>MACLSRIDANLLQYYEKPEPNNTVDLYVSNNSNNNGLKEGDKSISTPVPQPYGSEYSNCLLLSNSEYICYHFSSRSTLLTFYPLSDAYHGKTINIHLPNASMNQRYTLTIQEVEQQLLVNVILKDGSFLTLQLPLSFLFSSANTLNGEWFHLQNPYDFTVRVPHFLFYVSPQFSVVFLEDGGLLGLKKVDGVHYEPLLFNDNSYLKSLTRFFSRSSKSDYDSVISCKLFHERYLIVLTQNCHLKIWDLTSFTLIQDYDMVSQSDSDPSHFRKVEAVGEYLSLYNNTLVTLLPLENGLFQMGTLLVDSSGILTYTFQNNIPTNLSASAIWSIVDLVLTRPLELNVEASYLNLIVLWKSGTASKLQILNVNDESFKNYEWIESVNKSLVDLQSEHDLDIVTKTGDVERGFCNLKSRYGTQIFERAQQILSENKIIMAHNEDEEYLANLETILRDVKTAFNEASSITLYGDEIILVNCFQPYNHSLYKLNTTVENWFYNMHSETDGSELFKYLRTLNGFASTLSNDVLRSISKKFLDIITGELPDSMTTVEKFTDIFKNCLENQFEITNLKILFDELNSFDIPVVLNDLINNQMKPGIFWKKDFISAIKFDGFTSIISLESLHQLLSIHYRITLQVLLTFVLFDLDTEIFGQHISTLLDLHYKQFLLLNLYRQDKCLLAEVLLKDSSEFSFGVKFFNYGQLIAYIDSLNSNVYNASITENSFFMTFFRSYIIENTSHKNIRFFLENVECPFYLRHNEVQEFMFAMTLFSCGNFDQSYEIFQLHDYPEAINDKLPTFLEDLKSENYHGDSIWKDLLCTFTVPYRHSAFYYQLSLLFDRNNSQEFALKCISKSAEYSLKEIQIEELQDFKEKQHIHYLNLLIHFRMFEEVLDVLRLGHECLSDTVRTNFLQLLLQEDIYSRDFFSTLLRLCNAHSDNGELYLRTVDIKIVDSILSQNLRSGDWECFKKLYCFRMLNKSERAAAEVLYQYILMQADLDVIRKRKCYLMVINVLSSFDSAYDQWILNGSKVVTLTDLRDELRGL[2x];>MTIDDSNRLLMDVDQFDFLDDGTAQLSNNKTDEEEQLYKRDPVSGAILVPMTVNDQPIEKNGDKMPLKFKLGPLSYQNMAFITAKDKYKLYPVRIPRLDTSKEFSAYVSGLFEIYRDLGDDRVFNVPTIGVVNSNFAKEHNATVNLAMEAILNELEVFIGRVKDQDGRVNRFYELEESLTVLNCLRTMYFILDGQDVEENRSEFIESLLNWINRSDGEPDEEYIEQVFSVKDSTAGKKVFETQYFWKLLNQLVLRGLLSQAIGCIERSDLLPYLSDTCAVSFDAVSDSIELLKQYPKDSSSTFREWKNLVLKLSQAFGSSATDISGELRDYIEDFLLVIGGNQRKILQYSRTWYESFCGFLLYYIPSLELSAEYLQMSLEANVVDITNDWEQPCVDIISGKIHSILPVMESLDSCTAAFTAMICEAKGLIENIFEGEKNSDDYSNEDNEMLEDLFSYRNGMASYMLNSFAFELCSLGDKELWPVAIGLIALSATGTRSAKKMVIAELLPHYPFVTNDDIEWMLSICVEWRLPEIAKEIYTTLGNQMLSAHNIIESIANFSRAGKYELVKSYSWLLFEASCMEGQKLDDPVLNAIVSKNSPAEDDVIIPQDILDCVVTNSMRQTLAPYAVLSQFYELRDREDWGQALRLLLLLIEFPYLPKHYLVLLVAKFLYPIFLLDDKKLMDEDSVATVIEVIETKWDDADEKSSNLYETIIEADKSLPSSMATLLKNLRKKLNFKLCQAFM[2x];>MFNKSVNSGFTFGNQNTSTPTSTPAQPSSSLQFPQKSTGLFGNVNVNANTSTPSPSGGLFNANSNANSISQQPANNSLFGNKPAQPSGGLFGATNNTTSKSAGSLFGNNNATANSTGSTGLFSGSNNIASSTQNGGLFGNSNNNNITSTTQNGGLFGKPTTTPAGAGGLFGNSSSTNSTTGLFGSNNTQSSTGIFGQKPGASTTGGLFGNNGASFPRSGETTGTMSTNPYGINISNVPMAVADMPRSITSSLSDVNGKSDAEPKPIENRRTYSFSSSVSGNAPLPLASQSSLVSRLSTRLKATQKSTSPNEIFSPSYSKPWLNGAGSAPLVDDFFSSKMTSLAPNENSIFPQNGFNFLSSQRADLTELRKLKIDSNRSAAKKLKLLSGTPAITKKHMQDEQDSSENEPIANADSVTNIDRKENRDNNLDNTYLNGKEQSNNLNKQDGENTLQHEKSSSFGYWCSPSPEQLERLSLKQLAAVSNFVIGRRGYGCITFQHDVDLTAFTKSFREELFGKIVIFRSSKTVEVYPDEATKPMIGHGLNVPAIITLENVYPVDKKTKKPMKDTTKFAEFQVFDRKLRSMREMNYISYNPFGGTWTFKVNHFSIWGLVNEEDAEIDEDDLSKQEDGGEQPLRKVRTLAQSKPSDKEVILKTDGTFGTLSGKDDSIVEEKAYEPDLSDADFEGIEASPKLDVSKDWVEQLILAGSSLRSVFATSKEFDGPCQNEIDLLFSECNDEIDNAKLIMKERRFTASYTFAKFSTGSMLLTKDIVGKSGVSIKRLPTELQRKFLFDDVYLDKEIEKVTIEARKSNPYPQISESSLLFKDALDYMEKTSSDYNLWKLSSILFDPVSYPYKTDNDQVKMALLKKERHCRLTSWIVSQIGPEIEEKIRNSSNEIEQIFLYLLLNDVVRASKLAIESKNGHLSVLISYLGSNDPRIRDLAELQLQKWSTGGCSIDKNISKIYKLLSGSPFEGLFSLKELESEFSWLCLLNLTLCYGQIDEYSLESLVQSHLDKFSLPYDDPIGVIFQLYAANENTEKLYKEVRQRTNALDVQFCWYLIQTLRFNGTRVFSKETSDEATFAFAAQLEFAQLHGHSLFVSCFLNDDKAAEDTIKRLVMREITLLRASTNDHILNRLKIPSQLIFNAQALKDRYEGNYLSEVQNLLLGSSYDLAEMAIVTSLGPRLLLSNNPVQNNELKTLREILNEFPDSERDKWSVSINVFEVYLKLVLDNVETQETIDSLISGMKIFYDQYKHCREVAACCNVMSQEIVSKILEKNNPSIGDSKAKLLELPLGQPEKAYLRGEFAQDLMKCTYKI[2x];>MVVIANAHNELIHDAVLDYYGKRLATCSSDKTIKIFEVEGETHKLIDTLTGHEGPVWRVDWAHPKFGTILASCSYDGKVLIWKEENGRWSQIAVHAVHSASVNSVQWAPHEYGPLLLVASSDGKVSVVEFKENGTTSPIIIDAHAIGVNSASWAPATIEEDGEHNGTKESRKFVTGGADNLVKIWKYNSDAQTYVLESTLEGHSDWVRDVAWSPTVLLRSYLASVSQDRTCIIWTQDNEQGPWKKTLLKEEKFPDVLWRASWSLSGNVLALSGGDNKVTLWKENLEGKWEPAGEVHQ[2x];>[2x]MQPFDSGHDDLVHDVVYDFYGRHVATCSSDQHIKVFKLDKDTSNWELSDSWRAHDSSIVAIDWASPEYGRIIASASYDKTVKLWEEDPDQEECSGRRWNKLCTLNDSKGSLYSVKFAPAHLGLKLACLGNDGILRLYDALEPSDLRSWTLTSEMKVLSIPPANHLQSDFCLSWCPSRFSPEKLAVSALEQAIIYQRGKDGKLHVAAKLPGHKSLIRSISWAPSIGRWYQLIATGCKDGRIRIFKITEKNLQVELLSEHDDHNGEVWSVSWNLTGTILSSAGDDGKVRLWKATYSNEFKCMSVITAQQ;>MELSPTYQTERFTKFSDTLKEFKIEQNNEQNPIDPFNIIREFRSAAGQLALDLANSGDESNVISSKDWELEARFWHLVELLLVFRNADLDLDEMELHPYNSRGLFEKKLMQDNKQLYQIWIVMVWLKENTYVMERPKNVPTSKWLNSITSGGLKSCDLDFPLRENTNVLDVKDKEEDHIFFKYIYELILAGAIDEALEEAKLSDNISICMILCGIQEYLNPVIDTQIANEFNTQQGIKKHSLWRRTVYSLSQQAGLDPYERAIYSYLSGAIPNQEVLQYSDWESDLHIHLNQILQTEIENYLLENNQVGTDELILPLPSHALTVQEVLNRVASRHPSESEHPIRVLMASVILDSLPSVIHSSVEMLLDVVKGTEASNDIIDKPYLLRIVTHLAICLDIINPGSVEEVDKSKLITTYISLLKLQGLYENIPIYATFLNESDCLEACSFILSSLEDPQVRKKQIETINFLRLPASNILRRTTQRVFDETEQEYSPSNEISISFDVNNIDMHLIYGVEWLIEGKLYVDAVHSIIALSRRFLLNGRVKALEQFMERNNIGEICKNYELEKIADNISKDENEDQFLEEITQYEHLIKGIREYEEWQKSVSLLSSESNIPTLIEKLQGFSKDTFELIKTFLVDLTSSNFADSADYEILYEIRALYTPFLLMELHKKLVEAAKLLKIPKFISEALAFTSLVANENDKIYLLFQSSGKLKEYLDLVARTATLSN[2x];>[2x]MSEKKVHLRLRKELSVPIAVVENESLAQLSYEEESQASLMDISMEQQQLRLHSHFDNSKVFTENNRYIVKTLQTDYSSGFSNDDELNGYIDMQIGYGLVNDHKKVYIWNIHSTQKDTPYITVPFRSDDNDEIAVAPRCI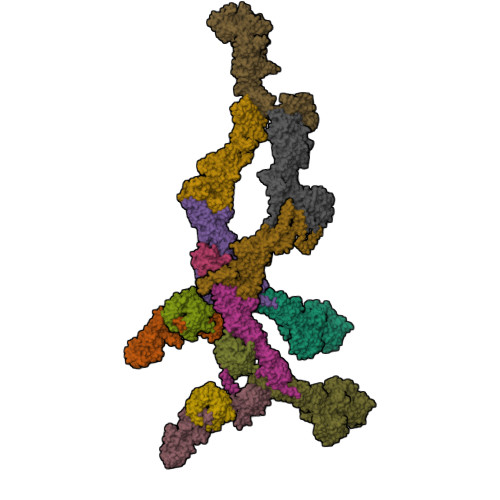LTFPATMDESPLALNPNDQDETGGLIIIKGSKAIYYEDINSINNLNFKLSEKFSHELELPINSSGGEKCDLMLNCEPAGIVLSTNMGRIFFITIRNSMGKPQLKLGKLLNKPFKLGIWSKIFNTNSSVVSLRNGPILGKGTRLVYITTNKGIFQTWQLSATNSHPTKLIDVNIYEAILESLQDLYPFAHGTLKIWDSHPLQDESSQLFLSSIYDSSCNETYYILSTIIFDSSSNSFTIFSTYRLNTFMESITDTKFKPKIFIPQMENANDTNEVTSILVMFPNAVVITQVNSKLDSSYSMRRKWEDIVSLRNDIDIIGSGYDSKSLYVLTKQMGVLQFFVKENEETNSKPEVGFVKSHVDQAVYFSKINANPIDFNLPPEISLDQESIEHDLKLTSEEIFHSNGKYIPPMLNTLGQHLSVRKEFFQNFLTFVAKNFNYKISPELKLDLIEKFEILNCCIKFNSIIRQSDVLNDIWEKTLSNYNLTQNEHLTTKTVVINSPDVFPVIFKQFLNHVVFVLFPSQNQNFKLNVTNLINLCFYDGILEEGEKTIRYELLELDPMEVDTSKLPWFINFDYLNCINQCFFDFTFACEEEGSLDSYKEGLLKIVKILYYQFNQFKIWINTQPVKSVNANDNFININNLYDDNHLDWNHVLCKVNLKEQCIQIAEFYKDLSGLVQTLQTLDQNDSTTVSLYETFFNEFPKEFSFTLFEYLIKHKKLNDLIFRFPQQHDVLIQFFQESAPKYGHVAWIQQILDGSYADAMNTLKNITVDDSKKGESLSECELHLNVAKLSSLLVEKDNLDINTLRKIQYNLDTIDAEKNISNKLKKGEVQICKRFKNGSIREVFNILVEELKSTTVVNLSDLVELYSMLDDEESLFIPLRLLSVDGNLLNFEVKKFLNALVWRRIVLLNASNEGDKLLQHIVKRVFDEELPKNNDFPLPSVDLLCDKSLLTPEYISETYGRFPIDQNAIREEIYEEISQVETLNSDNSLEIKLHSTIGSVAKEKNYTINYETNTVEY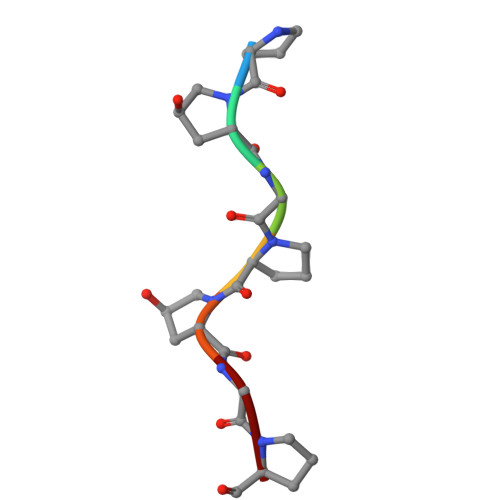> PPGPPGP>[2x]HHHHHHNKQVAMGRKKFNMDPKKGIQFLIENDLLKNTCEDIAQFLYKGEGLNKTAIG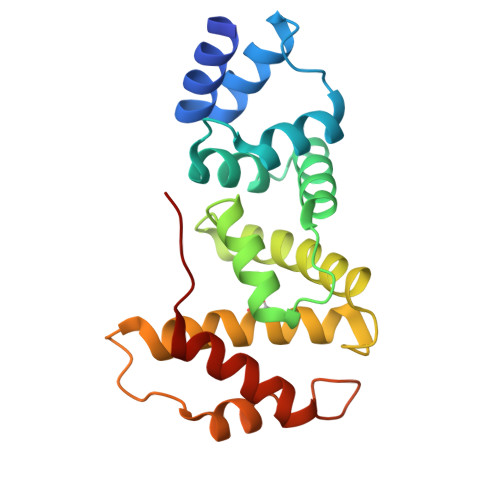DYLGERDEFNIQVLHAFVELHEFTDLNLVQALRQFLWSFRLPGEAQKIDRMMEAFAQRYCQCNNGVFQSTDTCYVLSFAIIMLNTSLHNPNVKDKPTVERFIAMNRGINDGGDLPEELLRNLYESIKNEPFKIPE> MVSRSMFDQLFKHRNSFYTYDAFIAAAKSFPSFGTTGDTDVRKREIAAFFAHVSHETSGGWPTAPDGPYAWGLVYIEEINQSNDYCDPSTQYPCAPGKQYYGRGPLQLSWNYNYGPCGDALGLDLLNNPDLVAQDPVIAFKTALWFWMTPQSPKPSCHDVMTGNWTPSSADLAAGRVPGFGVTTNIINGGLE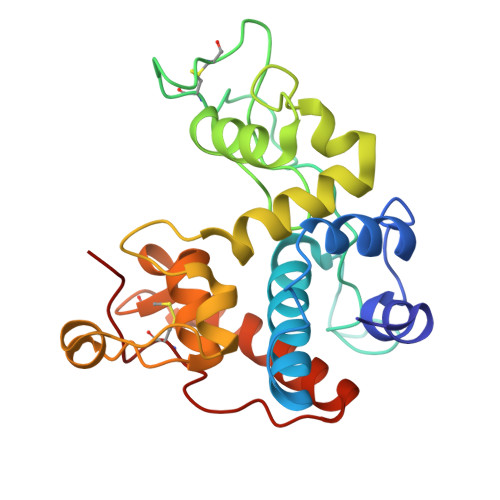CGKGNPAQAENRVNYYKDFCNQLGVSPGSNLDCANMRPFG> MDKELGKTLRRLRQGKQVSISSLADEHLSKSQISRFERGESEISCSRLLNLLDKLNITIDEFVSTHSKTHTHFFTLLSRVRKYYAEKNVAKLLKLLEDYAHKDYESTMIKAILSSIEPTVEPSEEEVTRLTDYLFSVEQWGYYEIILLGNCSRFINYNTLFLLTKEMVTSFAYSEQNKTNKTLVTQLSINCLIISIDYSYFDHSHYLIEKIEFLLRDELNF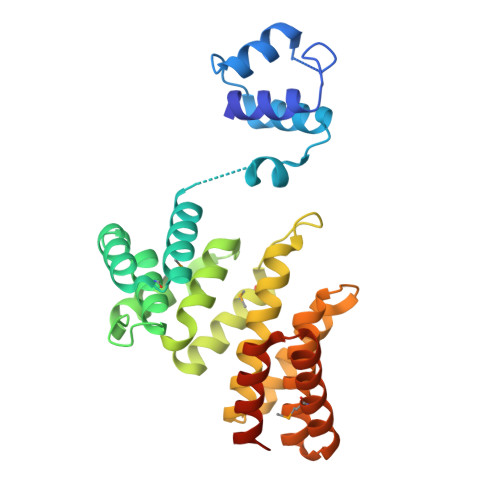YEKTVFLYVHGYYKLKQGQVSGKDDMRQALQIFKYLGEDALYYSYKEHYRKEVLGDEEDEEEG Aminoacyl-tRNA synthetases (aaRSs) catalyze the synthesis of aminoacyl-tRNAs, which are crucial building blocks for protein biosynthesis. Lysyl-tRNA synthetase (LysRS) has been validated as a promising target for antimalarial, anti-Cryptosporidium, anti-Pseudomonas aeruginosa, and anti-Mycobacterium tuberculosis therapies. The ATP-binding pocket is the most promising area for the development of LysRS inhibitors. We determined five cocrystal structures of LysRS in complex with the compounds in order to provide a basis for further optimization.

In comparison to compound 38, compound 36 has one more methoxy group substitution in the para position of the original 2-methoxy group. Compound 36 exhibited the highest PfLysRS binding affinity among these ASP3026 analogues. The ΔTm of PfLysRS induced by compound 36 was approximately 11.8 °C in the presence of l-lysine. The Kd value of compound 36 was 15.9 nM in SPR experiments, indicating stronger binding affinity than compound 38. Compound 36 also showed strong inhibition of PfLysRS enzyme activity in the ATP hydrolysis assay, with an IC50 of 198 nM, which was also stronger than ASP3026 in vitro. The ALK inhibitory ability of 36 was significantly reduced, and the IC50 was greater than 19.1 μM. To understand how these compounds are recognized by PfLysRS, we determined the cocrystal structures of PfLysRS with the compounds 34, 35, 36, and 38. The methoxy group inherited from ASP3026 in these compounds were all bound to the hydrophobic cavity formed by Arg330, Glu332, His338, Asn339, and Pro340 like ASP3026. The additional methoxy group of compound 36 formed a new H-bond with Arg330. Compound 36, in particular, exhibited the most potent inhibition with an EC50 value of 736 nM, surpassing the potency of ASP3026 by over sevenfold.

>[2x]MEVDPRLYFENRSKFIQDQKDKGINPYPHKFERTISIPEFIEKYKDLGNGEHLEDTILNITGRIMRVSASGQKLRFFDLVGDGEKIQVLANYSFHNHEKGNFAECYDKIRRGDIVGIVGFPGKSKKGELSIFPKETILLSACLHMLPMKYGLKDTEIRYRQRYLDLLINESSRHTFVTRTKIINFLRNFLNERGFFEVETPMMNLIAGGANARPFITHHNDLDLDLYLRIATELPLKMLIVGGIDKVYEIGKVFRNEGIDNTHNPEFTSCEFYWAYADYNDLIKWSEDFFSQLVYHLFGTYKISYNKDGPENQPIEIDFTPPYPKVSIVEEIEKVTNTILEQPFDSNETIEKMINIIKEHKIELPNPPTAAKLLDQLASHFIENKYNDKPFFIVEHPQIMSPLAKYHRTKPGLTERLEMFICGKEVLNAYTELNDPFKQKECFKLQQKDREKGDTEAAQLDSAFCTSLEYGLPPTGGLGLGIDRITMFLTNKNSIKDVILFPTMRPANGGHHHHHH> TVAYIAIGSNLASPLEQVNAALKALGDIPESHILTVSSFYRTPPLGPQDQPDYLNAAVALETSLAPEELLNHT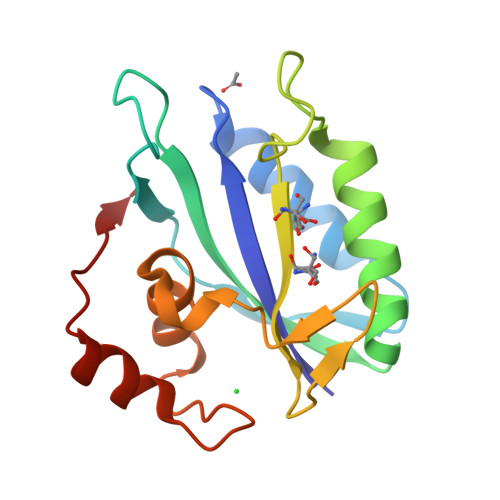QRIELQQGRVRKAERWGPRTLDLDIMLFGNEVINTERLTVPHYDMKNRGAMLWPLFEIAPELVFPDGEMLRQILHTRAFDKLNKW>[2x]MAHHHHHHMAASPEAKFT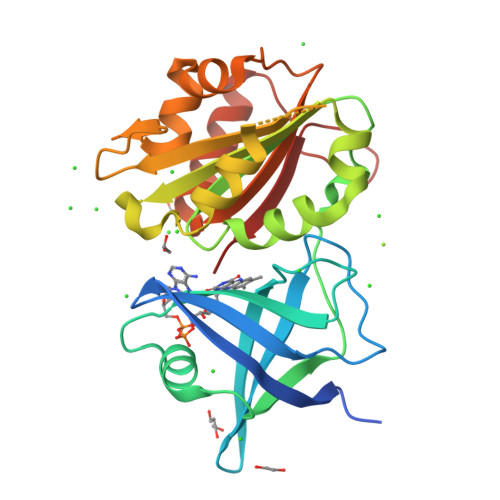EEKILWVKHHTPKLITFAISRPESYRFKAGQFSRLGFYEGKGFIWRAYSVVSAEYADTLEYFAVLIQDGPMSALFAKMQQGDTILLDKNATGFLLPERFPDGKDLVMLCTGSGIAPFLSILEQPEIRQRFDTVNLIHSVSFPEELIFNDRLAALSEHPLVGEYGHSFRFVPVTTRAANPSGLSGKRIPELLKNNSIEQALHTKLTPESTRFMICGNPEMVKDTFQTLLDMGYAMHRNRIPGQIMMENGF>GLSDWELAAARAAIARGLDEDLRYGPDVTTLATVPASATTTASLVTREAGVVAGLDVALLTLNEVLGTNGYRVLDRVEDGARVPPGEALMTLEAQTRGLLTAERTMLNLVGHLSGIATATAAWVDAVRGTKAKIRDTRKTLPGLRALQKYAVRTGGGVNHRLGLGDAALIKDNHVAAAGSVVDALRA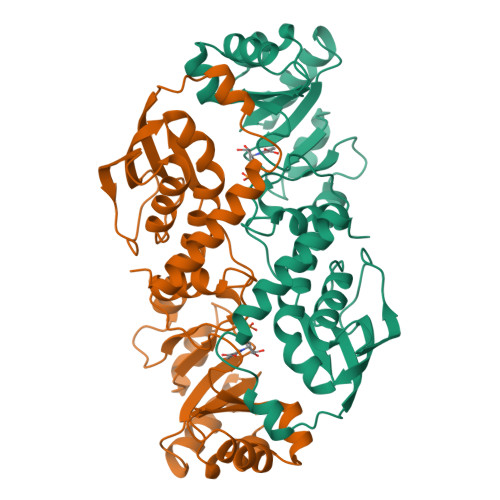VRNAAPDLPCEVEVDSLEQLDAVLPEKPELILLDNFAVWQTQTAVQRRDSRAPTVMLESSGGLSLQTAATYAETGVDYLAVGALTHSVRVLDIGLDM[6x]The AlkD/YtkR2/C10R5 enzymes belong to one of two known bacterial DNA glycosylase superfamilies that have evolved a non-base-flipping mechanism as a means to remove structurally diverse duplex-stabilizing adducts. By contrast, the BER pathway removes small nucleobase adducts, and is initiated by lesion-specific DNA glycosylases that hydrolyze the N-glycosidic bond to liberate the aberrant nucleobase from the DNA backbone. To understand AlkD’s lack of specificity for the three SCPCHD sub-types and comparatively high product affinity, we determined crystal structures of AlkD bound to DNA containing each of the three adducts. We previously showed that AlkD’s low level of protection against YTM results from product inhibition in which the enzyme remains bound to the newly formed abasic site in the DNA, slowing multiple-turnover excision, as well as impeding subsequent repair steps in the BER pathway.

Product complexes were generated by incubating AlkD with the corresponding DNA substrates, allowing for enzymatic hydrolysis of the N-glycosidic bond and formation of an AP site and a free nucleobase adduct. The conformations of AlkD and the abasic DNA are effectively identical in the three structures. Within the SCPCHD binding cleft, 14 protein residues contact one or more of the adducts. Only three—Gln38, Lys156, and Lys194—form adduct-specific hydrogen-bonding interactions. Gln38 interacts with the hydroxyl and methoxy substituents of the S−1 subunit unique to YTM, while Lys194 interacts with the methoxy substituent of the S+2 subunit unique to CC-1065. Lys156 contacts all three adducts but only forms a hydrogen-bonding interaction with the hydroxyl substituent specific to the S+1 subunit of CC-1065. YtkR2 also provided significant resistance against CC-1065, which was somewhat unexpected because of the presence of the unique S+2 subunit, and suggests that interactions with this subunit do not play an important role in determining substrate specificity. Indeed, the outward face of the S+2 subunit is largely solvent exposed and has the fewest protein contacts of any subunit. Thus, AlkD’s substrate-binding cleft can accommodate each SCPCHD compound with strikingly few adduct-specific interactions.

> GPVPMHPFVKALQEHFTAHQNPEKAEPMARYMKNHFLFLGIQTPERRQLLKDIIQIHTLPDQKDFQIIIRELWDLPEREFQAAALDIMQKYKKHINETHIPFLEELIVTKSWWDSVDSIVPTFLGDIFLKHPELISAYIPKWIASDNIWLQRAAILFQLKYKQKMDEELLFWIIGQLHSSKEFFIQKAIGWVLREYAKTNPDVVWEYVQNNELAPLSKREAIKHIKQNYGINNEKIGETLS>MSSASSNARDEVIAAIHEEADWVDRTVYPFESRCIGLSSGAVHYIDEGPDDGGRETLLMLHGNPTWSFLYRHLVRDLRDEYRCVALDYLGFGLSERPTDFSYRPEDHADVVEEFIDELGLEDVVLVGHDWGGPIGFSYAIDHPENVGGLVVMNTWMWPVSDDKHFSRFSKLLRIGRELCERYDLFTRVIMPMGFADRSRFTESAREQYRAANRGDRTGTGIFPQAILGSRAWLSSLWEQRDNIADIPARIIWGMEDSAFRPAELRTFEALFEDSSTVRLYGVGHYVPEEFGSDLVPLVREFLEEVHHHHHH[10x]

Haloalkane dehalogenases (EC 3.8.1.5, HLDs) are a group of enzymes that catalyze the hydrolytic cleavage of a carbon–halogen bond in a range of halogenated organic compounds. Here we probe the structural organization of DhmeA, a subfamily III HLD‐like enzyme from the archaeon Haloferax mediterranei, by combining cryo‐electron microscopy (cryo‐EM) and x‐ray crystallography. A distinct catalytic pentad forms the active site of HLD enzymes: a nucleophile aspartic acid, a histidine base, a catalytic acid (aspartic or glutamic acid) and two halide stabilizing residues (two tryptophans or tryptophan + asparagine) (Janssen, 2004). We show that full‐length wild‐type DhmeA forms diverse quaternary structures, ranging from small oligomers to large supramolecular ring‐like assemblies of various sizes and symmetries.

We noted that the solvent‐exposed L10 loop, connecting α4 and α5' helices in the cap domain, displays a unique feature containing two glycine residues (G173, G174) in DhmeA. We thus constructed a DhmeA mutant lacking these two glycines, hereafter referred to as DhmeA∆GG. Importantly, the DhmeA∆GG protein could be reproducibly crystallized. The final model contains 10 DhmeA molecules in the asymmetric unit and has a low deviation from the ideal geometry. The 3.3 Å crystal structure reveals that DhmeAΔGG forms a ring‐like 20‐mer structure with outer and inner diameter of ~200 and ~80 Å, respectively. The crystallographic ring contains three types of assembly interfaces, namely di‐, tetra‐, and multimerization interface. An unusual striking feature of the DhmeAΔGG organization is that the first monomeric unit in the homodimer has a complete, properly folded helical cap domain, while the cap domain of the second monomeric unit is partially unfolded and distorted. Notably, the electron density map between residues R181 and D196, encompassing α5′ and α5 helices, is missing, and this part could not be built into the model. Therefore, we suggest that the cap domain of DhmeA protein may naturally unfold, which leads to an uncovering of the active site. The exterior of the ring together with the multimerization interface has a highly negatively charged surface, while the interior is decorated with a positive charge with the highest positive surface charge density around the tetramerization interface.> GSHMLTPTLVSLLEVIEPEVLYAGYDSSVPDSTWRIMTTLNMLGGRQVIAAVKWAKAIPGFRNLHLDDQMTLLQYSWMSLMAFALGWRSYRQSSANLL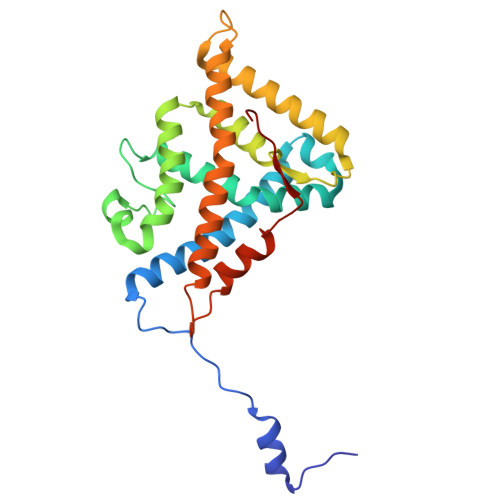CFAPDLIINEQRMTLPDMYDQCKHMLYVSSELHRLQVSYEEYLCMKTLLLLSSVPKDGLKSQALFDAIRMTYIKELGKAIVKREGNSSQNSQRFYQLTKLLDSMHEVVENLLNYCFQTFLDKTMSIEFPEMLAEIITNQIPKYSNGNIKKLLFHQK>[3x]MSNLPVEPEFEQAYKELASTLENSTLFQKNPEYRKALAVVSVPERVIQFRVVWENDKGEVQVNRGFRVQFNSALGPYKGGLRFHPSVNLSILKFLGFEQIFKNALTGLNMGGGKGGSDFDPKGKSDSEIRRF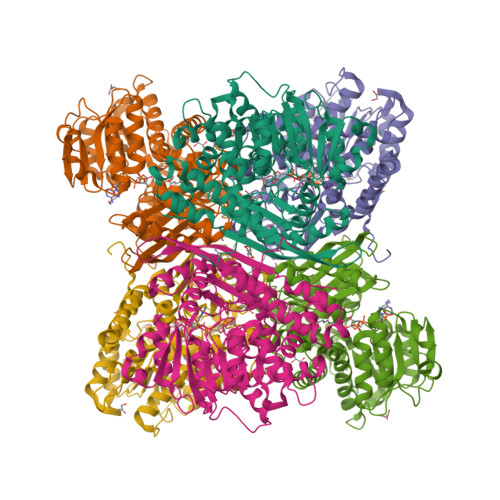CVAFMTELCRHIGADTDVPAGDIGVTGREIGYLFGQYRKLRNSWEGVLTGKGGSWGGSLIRPEATGYGVVYYVEHMIAHATNGAESFAGKRVAISGSGNVAQYAALKVIELGGRVVSLSDSQGSLIVKDTAKDSFTPAEIDAIAALKVDRKQIAELVTDAAFADKFTYLPGQRPWVHVGAVDVALPSATQNEVSGEEAQALIAAGCKFIAEGSNMGCTQAAIDAFEAHREANKGAAAIWYAPGKAANAGGVAVSGLEMAQNSARLSWTAEEVDARLKDIMKSCFQNGLDTAKEYATPADGILPSLVTGSNIAGFTKVAAAMKDQGDWW>[6x]SGLENIAFNVVNKGSFVSADGELPVAISGDKVFVRDGNTDNLVFVNKTSLPTNIAFELFAKRKVGLTPPLSILKNLGVVATYKFVLWDYEAERPLTSFTKSVCGYTDFAEDVCTCYDNSIQGSYERFTLSTNAVLFSATAVKAGGKSLPAIKLNFGMLNGN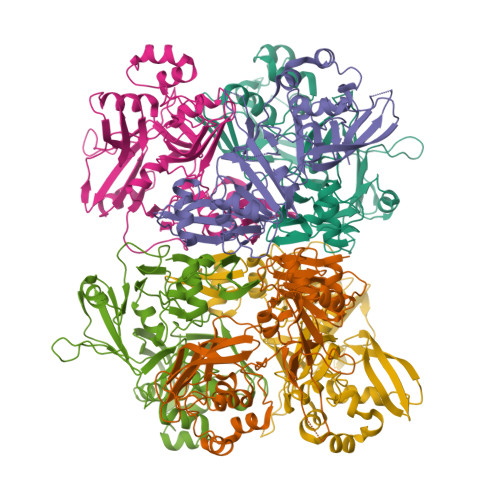AIATVKSEDGNIKNINWFVYVRKDGKPVDHYDGFYTQGRNLQDFLPRSTMEEDFLNMDMGVFIQKYGLEDFNFEHVVYGDVSKTTLGGLHLSISQVRLSKMGILKAEEFVAASDITLKCCTVTYLNDPSSKTVCTYMDLLLDDFVSVLKSLDLTVVSKVHEVIIDNKPWRWMLWCKDNAVATFYPQLQ3-sialyllactose | C23 H39 N O19 | 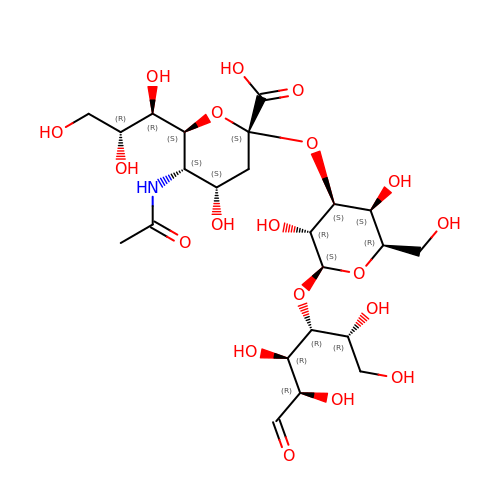OIZGSVFYNBZVIK-KYPQSLRHSA-N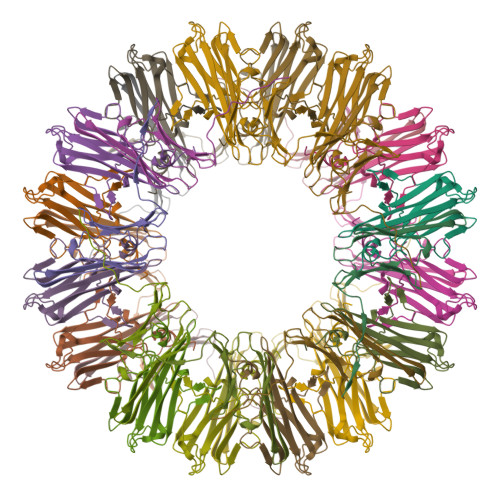>[4x]MSSLCPYTGRPTGLFRDFEDMMPYWAQRHSMLNNFNNIVPQQLNEVENTAQKFCVKLDVAAFKPEELKVNLEGHVLTIEGHHEVKTEHGFSKRSFTRQFTLPKDVDLAHIHTVINKEGQMTIDAPKTGSNTTVRALPIHTSAGHAVTQKPSSTTTTGKH2,3-dihydro-1,4-benzodioxine-5-carboxylic 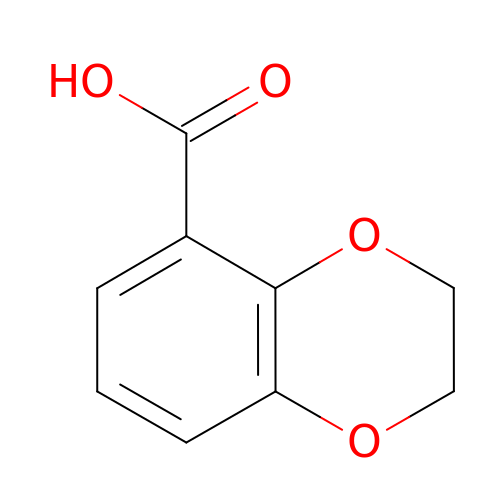acid | C9 H8 O4 | VCLSWKVAHAJSFL-UHFFFAOYSA-N>MKEVEVLMETKNTQSPQTPLVEPVTERTKLQEHTIFTQLKKNIPKTRYNRDYMLSMANIPERIINVGVIGPLHSGKTSLMDLLVIDSHKRIPDMSKNVELGWKPLRYLDNLKQEIDRGLSIKLNGSTLLCTDLESKSRMINFLDAPGHVNFMDETAVALAASDLVLIVIDVVEGVTFVVEQLIKQSIKNNVAMCFVINKLDRLILDLKLPPMDAYLKLNH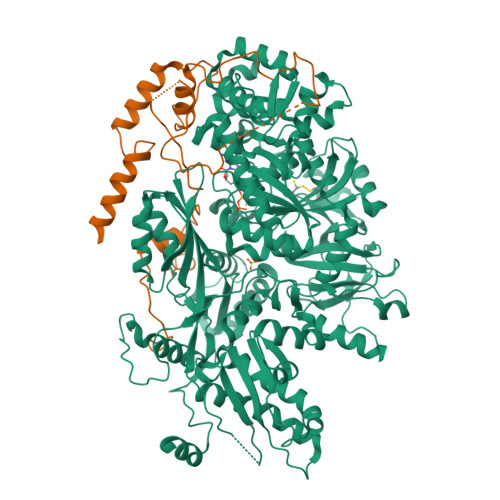IIANINSFTKGNVFSPIDNNIIFASTKLGFTFTIKEFVSYYYAHSIPSSKIDDFTTRLWGSVYYHKGNFRTKPFENVEKYPTFVEFILIPLYKIFSYALSMEKDKLKNLLRSNFRVNLSQEALQYDPQPFLKHVLQLIFRQQTGLVDAITRCYQPFELFDNKTAHLSIPGKSTPEGTLWAHVLKTVDYGGAEWSLVRIYSGLLKRGDTVRILDTSQSESRQKRQLHDISKTETSNEDEDEDDETPSCEVEEIGLLGGRYVYPVHEAHKGQIVLIKGISSAYIKSATLYSVKSKEDMKQLKFFKPLDYITEAVFKIVLQPLLPRELPKLLDALNKISKYYPGVIIKVEESGEHVILGNGELYMDCLLYDLRASYAKIEIKISDPLTVFSESCSNESFASIPVSNSISRLGEENLPGLSISVAAEPMDSKMIQDLSRNTLGKGQNCLDIDGIMDNPRKLSKILRTEYGWDSLASRNVWSFYNGNVLINDTLPDEISPELLSKYKEQIIQGFYWAVKEGPLAEEPIYGVQYKLLSISVPSDVNIDVMKSQIIPLMKKACYVGLLTAIPILLEPIYEVDITVHAPLLPIVEELMKKRRGSRIYKTIKVAGTPLLEVRGQVPVIESAGFETDLRLSTNGLGMCQLYFWHKIWRKVPGDVLDKDAFIPKLKPAPINSLSRDFVMKTRRRKGISTGGFMSNDGPTLEKYISAELYAQLRENGLVPWSHPQFEK[2x];>[2x]MWSHPQFEKSTPLRDEVTDKNYYYLFDKKSFFNGKALNNAIPGGPKFEPLYPREEEEDYNEFNSIDRVIFRVPIRSEYKVAFPHLYNSRPRSVRIPWYNNPVSCIIQNDEEYDTPALFFDPSLNPIPHFIDNNSSLNVSNTKENGDFTLPEDFAPLLAEEEELILPNTKDAMSLYHSPFPFNRTKGKMVRAQDVALAKKWFLQHPDEEYPVKVKVSYQKLLKNYVLNELHPTLPTNHNKTKLLKSLKNTK>GHMKTSKWIDISQPLNNDIATWPGDTPFSYEVLWSKEESGSVNVGKLTMSIHTGTHIDAPFHFDNDGKKVLDLDIQVYVGPTRIIDVSNLESIGKKELEKFHLEGVERLLLRTSSHGKANEFPDIIPHLRADIAPFLSEKGIRLIGVDVPSVDPLDDKELAAHHQLFKHSIHILENVVLDHVADGDYELIALPLALSDADGSPVRAVIRPI[4x]

The proteins involved in tryptophan catabolism are in general highly conserved across species, but with the notable exception of the second enzyme in the pathway: kynurenine formamidase. This enzyme catalyses the conversion of N-formyl-L-kynurenine (NFK) into formate and L-kynurenine. Our attention was drawn to the prokaryotic KFase KynB (EC 3.5.1.9). The KynB subunit, approximate mass 23 kDa, comprises just over 200 residues with about 50% in 12 β-strands and 15% in four α-helices.

A structure was required without Cd2+ being present, or indeed any transition metal ions other than Zn2+ and for which we could obtain data to inform on substrate recognition. Highly ordered structures of BaKynB and a complex with 2-aminoacetophenone at resolutions of 1.9 and 2.3 Å resulted and confirmed the binuclear Zn2+ environment. The enzyme active site is a narrow cavity approximately 7 Å×12 Å and 10 Å in depth, lined by hydrophobic walls composed of Trp20, His60 and Leu158 from one subunit, and Val40 and Val42 from the partner. At the base of the cavity is a polar floor, where two Zn2+ ions, separated by a distance of 3.1 Å, are bound. One Zn2+ is co-ordinated by Asp56, His161, Glu173 and a water molecule/hydroxide ion in a tetrahedral fashion with distances less than 2.3 Å. The water/hydroxide co-ordinates with the other cation and acts as a bridge for the binuclear site. In a similar fashion, the other cation also has four ligands co-ordinating with distances less than 2.3 Å. These are His50, His54, Asp56 and the bridging water/hydroxide. Furthermore, unlike other metallohydrolases where conformational flexibility appears to be important, the catalytic site of KynB is relatively rigid with an average thermal parameter (B-factor) of 9.6 Å2 compared with an overall average of 15.1 Å2 in BaKynB.>MGRRRSHERRDLPPNLYIRNNGYYCYRDPRTGKEFGLGRDRRIAITEAIQANIELFSGHKHKPLTARINSDNSVTLHSWLDRYEKILASRGIKQKTLINYMSKIKAIRRGLPDAPLEDITTKEIAAMLNGYIDEGKAASAKLIRSTLSDAFREAIAEGHITTNHVAATRAAKSEVRRSRLTADEYLKIYQAAESSPCWLRLAMELAVVTGQRVGDLCEMKWSDIVDGYLYVEQSKTGVKIAIPTALHIDALGISMKETLDKCKEILGGETIIASTRREPLSSGTVSRYFMRARKASGLSFEGDPPTFHELRSLSARLYEKQISDKFAQHLLGHKSDTMASQYRDDRGREWDKIEIK[4x];>ALTKAEMSEYLFDKLGLSKRDAKELVELFFEEIRRALENGEQVKLSGFGNFDLRDKNQRPGRNPKTGEDIPITARRVVTFRPGQKLKSRVENASPK[2x];>[2x]MTKSELIERLATQQSHIPAKTVEDAVKEMLEHMASTLAQGERIEIRGFGSFSLHYRAPRTGRNPKTGDKVELEGKYVPHFKPGKELRDRANIYG;>[3x]MYLTLQEWNARQRRPRSLETVRRWVRESRIFPPPVKDGREYLFHESAVKVDLNRP

The site-specific recombinase (Int) encoded by bacteriophage λ is the archetypical member of the tyrosine recombinase family, whose members carry out such diverse functions as chromosome segregation, chromosome copy number control, gene expression, conjugative transposition, gene dissemination, and viral integration and excision. All tyrosine recombinases use the same isoenergetic phosphoryl transfer chemistry and sequential strand exchange mechanism to execute DNA rearrangements via the formation and resolution of a transient four-way DNA junction, or Holliday junction (HJ), recombination intermediate. Int is a heterobivalent DNA binding protein that binds to high affinity 'arm-type' DNA sites via its small amino-terminal domain (NTD) and more weakly to 'core-type' DNA sites, where DNA cleavage and ligation take place. The Int subunits within a recombinogenic complex bind and bridge arm- and core-type DNA sites in patterns determined by the accessory DNA bending proteins IHF, Xis, and Fis.

Using techniques described previously, we trapped and purified the multi-protein HJ complex of excisive recombination and determined its structure at 11 Å resolution using single particle electron cryo-microscopy (cryo-EM). At the center of the excisive complex an integrase tetramer is bound to a core-site HJ, where strand exchange has taken place between the B half-site of attL and the C half-site of attR. IHF heterodimers bend the P arm at the H2 site and the P' arm at the H' site, in each case re-directing the DNA back towards the Int tetramer. For P', the IHF bend is sufficient for the P'1 and P'2 arm-binding sites to be engaged by the Int subunits bound at the C' and B core sites, respectively. A sharp IHF (yellow) directed bend at the H2 site, combined with the cooperative binding and bending by three Xis molecules (gold) and the Int subunit bridging between the B' and P2 sites (magenta), redirects the P arm over the top of the Int tetramer. As a result of the IHF and Xis-induced bends, the P2 site is positioned where it can be engaged by the Int subunit bound to the B' core site. The EM structure reveals that Xis also mediates a substantial protein-protein interface between the P and P' arms. The Xis molecules bound at the X1 and X1.5 sites of the P arm are packed against the Int-B and Int-C' NTDs bound at the P'2 and P'1 sites, respectively. Instead, Xis-NTD, and possibly Xis-linker interactions provide the additional glue required to hold attL and attR together and allow the initial strand exchange to take place. The core HJ isomer that we fit in the EM structure corresponds to a bottom strand cleavage configuration, where the complex is poised to carry out strand exchange to form attP and attB products.>SMALLQVTISLSKVELSVGESKFFTCTAIGEPESIDWYNPQGEKIISTQRVVVQKEGVRSRLTIYNANIEDAGIYRCQATDAKGQTQEATVVLEIYQKLTFREVVSPQEFKQGEDAEVVCRVSSSPAPAVSWLYHNEEVTTISDNRFAMLANNNLQILNINKSDE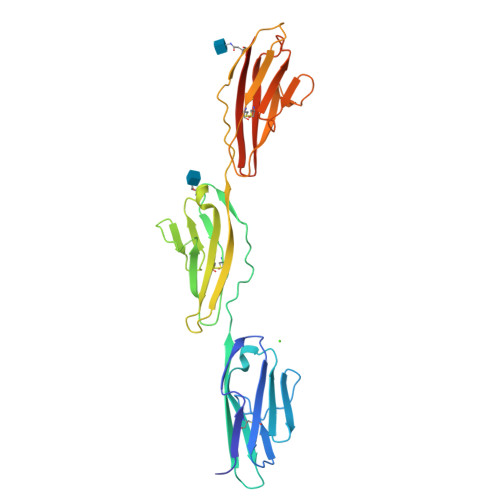GIYRCEGRVEARGEIDFRDIIVIVNVPPAISMPQKSFNATAERGEEMTFSCRASGSPEPAISWFRNGKLIEENEKYILKGSNTELTVRNIINSDGGPYVCRATNKAGEDEKQAFLQVFVQHHHHHH[2x]1-S-(carboxymethyl)-1-thio-beta-D-fructopyranose | C8 H14 O7 S | 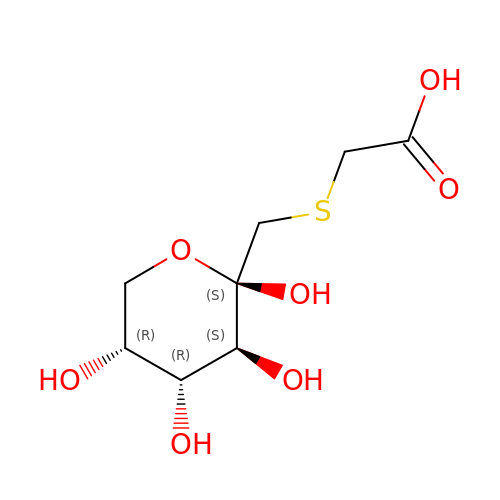UORIXTGMSRMKDZ-CCXZUQQUSA-N>[4x]ADGKAIFQQKGCGSCHQANVDTVGPSLKKIAQAYAGKEDQ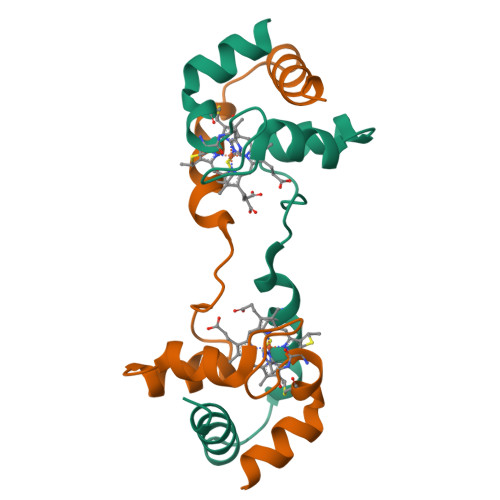LIKFLKGEAPAIVDPAKEAIMKPQLTMLKGLSDAELKALADFILSHK> MKASTVLQIAYLVSQESKCCSWKVGAVIEKNGRIISTGYNGSPAGGVNCCDYAAEQGWLLNKPKHAIIQGHKPECVSFGSTDRFVLAKEHRSAHSEWSSKNEIHAELNAILFAAENGSSIEGATMYVTLSPCPDCAKAIAQSGIKKLVYCETYDKNKPGWDDILRNAGIEVF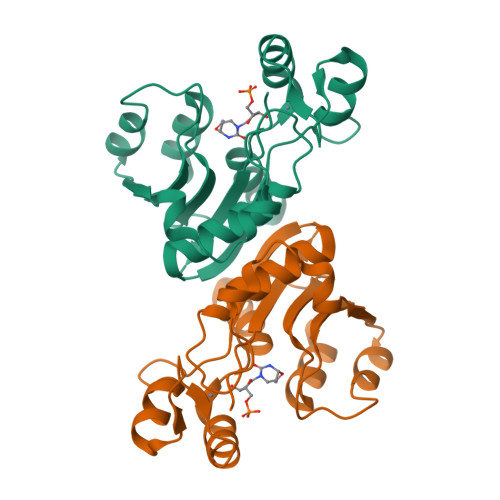NVPKKNLNKLNWENINEFCGE>SMITKETKTIGVLVPDITNPFFSTLMRGIEDILYKQNFVTILCNADSDHQKEIEYLAELTRRGVDGFIIATSAVSTDAINENLKKQGRPFIVLDQKKSEGFSDAVRTDDFRGGYLAGMHLLSLGHQTIALVYPENPPENVHARIEGFKSALDVYQIPHDQLILLPTQFSKQGGYQITAELLDSAATGVFALNDELAFGLYRGLEEAGKSIPEDYSIIGYDNIDMCEYIKPKLTTIAQPIFELGQTSA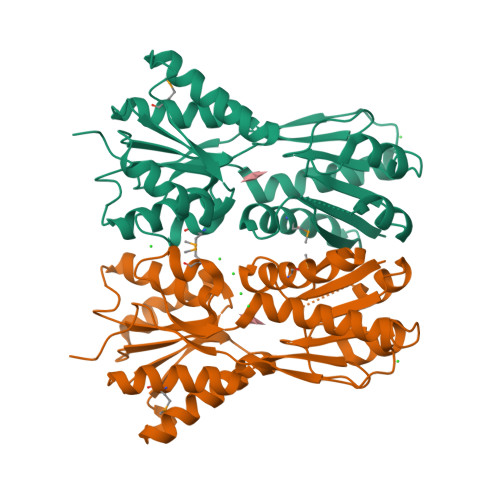KLLLDRIQFPEKEWEEKRLPVRFEKRFSTAPLK[6x]>[2x]MDGAGAEEVLAPLRLAVRQQGDLVRKLKEDKAPQVDVDKAVAELKARKRVLEAKELALQPKDDIVDRAKMEDTLKRRFFYDQAFAIYGGVSGLYDFGPVGCALKNNIIQTWRQHFIQEEQILEIDCTMLTPEPVLKTSGHVDKFADFMVKDVKNGECFRADHLLKAHLQKLMSDKKCSVEKKSEMESVLAQLDNYGQQELADLFVNYNVKSPITG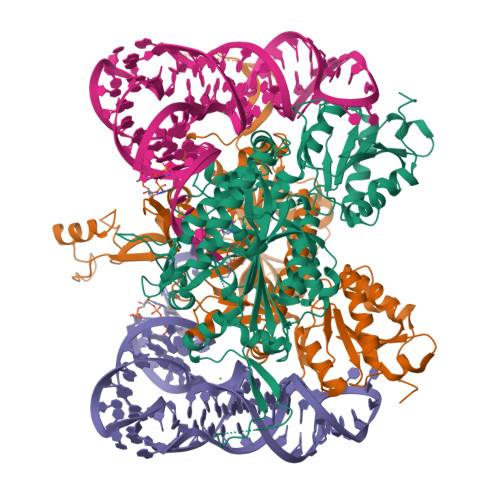NDLSPPVSFNLMFKTFIGPGGNMPGYLRPETAQGIFLNFKRLLEFNQGKLPFAAAQIGNSFRNEISPRSGLIRVREFTMAEIEHFVDPSEKDHPKFQNVADLHLYLYSAKAQVSGQSARKMRLGDAVEQGVINNTVLGYFIGRIYLYLTKVGISPDKLRFRQHMENEMAHYACDCWDAESKTSYGWIEIVGCADRSCYDLSCHARATKVPLVAEKPLKEPKTVNVVQFEPSKGAIGKAYKKDAKLVMEYLAICDECYITEMEMLLNEKGEFTIETEGKTFQLTKDMINVKRFQKTLYVEEVVPNVIEPSFGLGRIMYTVFEHTFHVREGDEQRTFFSFPAVVAPFKCSVLPLSQNQEFMPFVKELSEALTRHGVSHKVDDSSGSIGRRYARTDEIGVAFGVTIDFDTVNKTPHTATLRDRDSMRQIRAEISELPSIVQDLANGNITWADVEARYPLFEGQETGKKETIEELEHHHHHH>[2x]GMGLALCGAAAQAQEKPNFLIIQCDHLTQRVVGAYGQTQGCTLPIDEVASRGVIFSNAYVGCPLSQPSRAALWSGMMPHQTNVRSNSSEPVNTRLPENVPTLGSLFSESG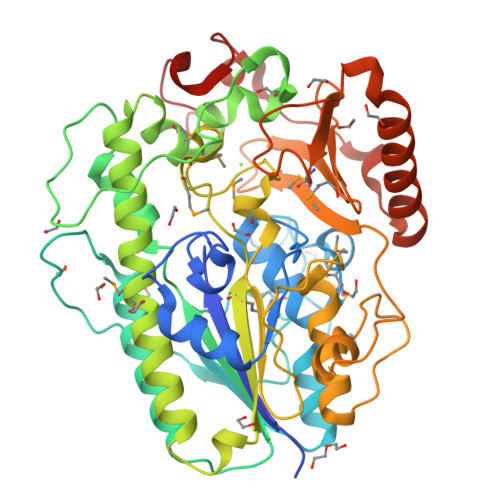YEAVHFGKTHDMGSLRGFKHKEPVAKPFTDPEFPVNNDSFLDVGTCEDAVAYLSNPPKEPFICIADFQNPHNICGFIGENAGVHTDRPISGPLPELPDNFDVEDWSNIPTPVQYICCSHRRMTQAAHWNEENYRHYIAAFQHYTKMVSKQVDSVLKALYSTPAGRNTIVVIMADHGDGMASHRMVTKHISFYDEMTNVPFIFAGPGIKQQKKPVDHLLTQPTLDLLPTLCDLAGIAVPAEKAGISLAPTLRGEKQKKSHPYVVSEWHSEYEYVTTPGRMVRGPRYKYTHYLEGNGEELYDMKKDPGERKNLAKDPKYSKILAEHRALLDDYITRSKDDYRSLKVDADPRCRNHTPGYPSHEGPGAREILKRK> SFFYDRSTLSSVLQSTSDVSSKFTPSTAKNLQNSILLTPLPSDIVNNSVLPEQERWISFASPTTQKPPYKTKQDWNFIMFSPFTYYKCDLEVTLSKNDRETISSVVRYVPCGAPSDLSDQTMPQTPSLADTRDPHMWVVGQGTTNQISFVIPYTSPLSVLPSVWFNGFSNFDNSSRFGVAPNADFGRLLLQGQGTFSVHYRYKKMRVFCPRPTVFIPWP;> LLSLCKIPTFLGNLDSNKKRIPYFSATNSTPATPLVTYQVTLSCSCMANSMLAAVARNFNQYRGSLNYLFVFTGSAMTKGKFLISYTPPGAGEPKTLDQAMQATYAIWDLGLNSSYNFTVPFISPTHYRQTSYNTPTITSVDGWLTVWQLTPLTYPLGVPNDSHILTLVSGGDDFTLRMPVTFTKYVPQ;> SDRVSSDTAGNTATNTQSTVGRLFGFGQRHKGKHPASCADTATDKVLAAERYYTIKLASWTKTQESFDHIRVPLPHALAGENGGVFSSTLRRHYLCKCGWRIQVQCNASQFHAGSLLVFMAPEFDTSNHSTEVEPRADTAFKVDANWQKHAQILTGHAYVNTTTKVNVPLALNHQNFWQWTTYPHQILNLRTNTTCDLEVPYVNVCPTSSWTQHANWTLVIAVLTPLQYSQGSATTIEITASIQP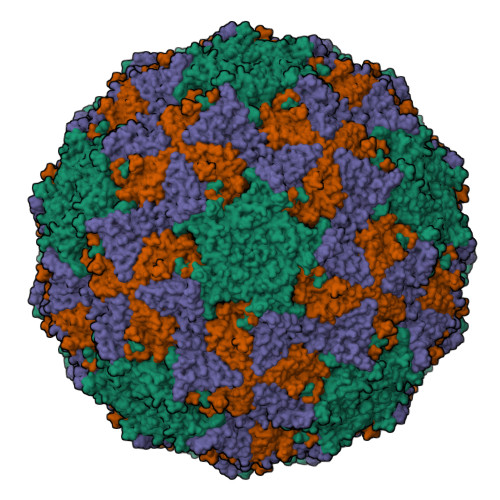VKPVFNGLRHTVV> SNAMVHAVTGGQPPSEAQVRQAAWIARCVGRGGSAPLHRDDVSALAETLQVKEFAPGAVVFHADQTADGVWIVRHGLIELAVGSRRRRAVVNILHPGDVDGDIPLLLEMPMVYTGRALT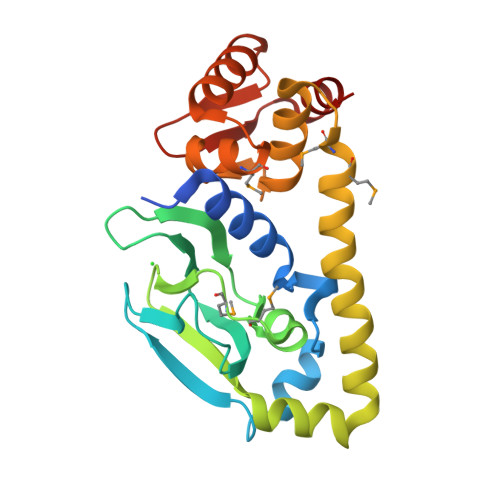QATCLFLDRQAFERLLATHPAIARRWLSSVAQRVSTAQIRLMGMLGRPLPAQVAQLLLDEAIDARIELAQRTLAAMLGAQRPSINKILKEFERDRLITVGYAVIEITDQHGLRARAQ> NNEIMPGKMKVKATKGEGDGGITSEGNALYNNEGG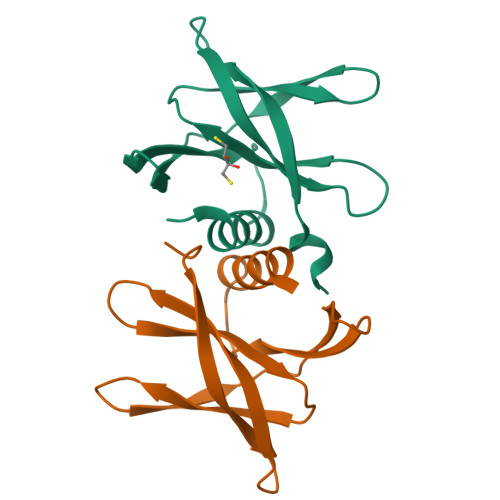RAFMYAYVTTKPGMKYVKWEHDSGVVTVELEPPARFVIDTPTGPQIKYLYFVKNLNNLRRGAVLGYIGATVRLQ;> NNEIKPGKMKVKATKGEGDGGITSEGNALYNNEGGRAFMYAYVTTKPGMKYVKWEHDSGVVTVELEPPARFVIDTPTGPQIKYLYFVKNLNNLRRGAVLGYIGATVRLQ> MLKRNARQPKALKVSTGPTLYGLMAEFDDAEALLAAAEKTRDAGYKQFEAYTPMPIHGLDEAVGYRGTRLPWVIFGAGLLGASGMFALQ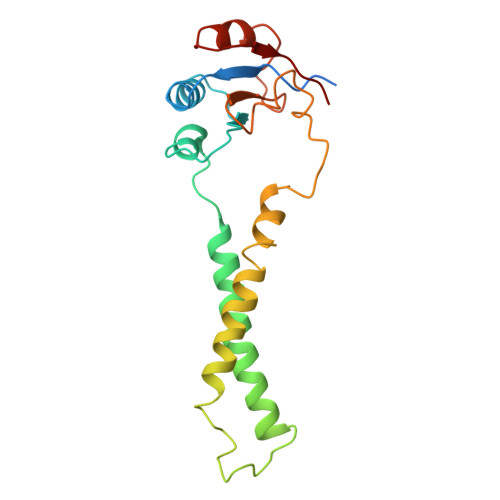TWINLVEYPLNIGGRPLFSWPAFIPATFEGMVLLSAFAAVFGMIAACGLPRPYHPVFNAPNFERASVDRFFLCIEAADPKFELKQTRQFLESLGPLAVSTVDN> HMASMKKKGSVVIVGRINLSGDTAYAQQTRGEEGCQETSQTGRDKNQ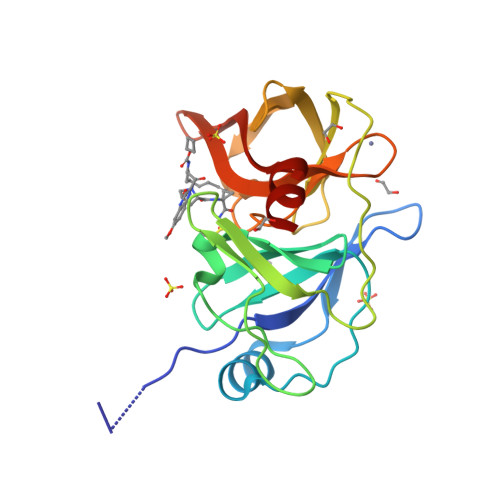VEGEVQIVSTATQTFLATSINGVLWTVYHGAGTRTIASPKGPVTQMYTNVDKDLVGWQAPQGSRSLTPCTCGSSDLYLVTRHADVIPVRRRGDSRGSLLSPRPISYLKGSSGGPLLCPAGHAVGIFRAAVSTRGVAKAVAFIPVESLETTSRS>[8x]MPVTNLAELDALVARVKAAQAEFATFSQEQVDKIFRAASLAANQARIPLAQMAVEESGMGIVEDKVIKNHFASEFIYNKYKDEKTCGILEEDDNLGTMTIAEPVGIICGIVPTTNPTSTAIFKSLISLKTRNGIIFSPHPRAKNSTNAAAKLVLDAAIAAGAPKDIIGWIDQPSVELSNALMKHDGIALILATGGPGMVKAAYSSGKPAIGVGAGNVPVVIDETADIKRAVASILMSKTFDNGVVCASEQAAIVVSEVYDEVKERFATHKAHVLSKA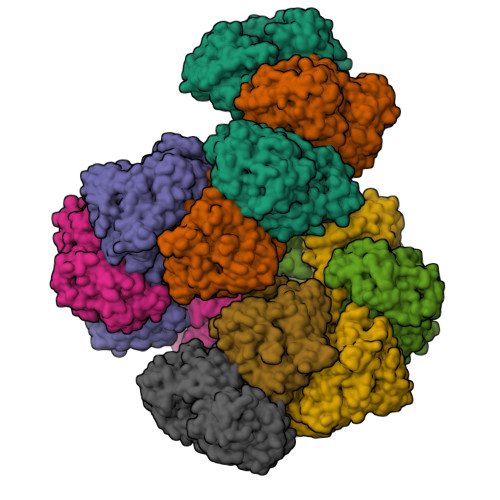DADKVRKVLLIDGALNAKIVGQPAAAIAEMAGVKVPADTKVLVGEGLGKVSYDDEFAHEKLSPTLGLFRADNFEDAVAQAVTMVEIGGIGHTSGLYTNQDVNADRIRYFGDKLKTARILVNIPTTHGGIGDLYNFNVAPSLTLGCGSWGGNSISENVGPKHLINKKTVAKRAENMLWHKLPKSIYFRRGSLPIALSDLEGKKRAFLVTDRFLFNNGYADDVVALLKAQGMEVQTFFEVEADPTLSVVEKGAAAMQSFQPDVILALGGGSPMDAAKIMWVMYEHPDTHFEELAMRFMDIRKRIYKFPKMGKKAELVCITTTSGTGSEVTPFAVVTDDKTGAKYPLADYELTPQMAIVDANLVMNMPKSLTAFGGYDAVTHALEAYVSVLANEYSDGQALQALKMLKEYLPSSYANGAKDPIAREKVHNAATIAGIAFANAFLGVCHSMAHKIGAEFHLPHGLANALLIANVVRYNANDNPTKQTAFSQYDRPQARRRYAEVADHLGLSQPGDRTAQKIERLLTWLDELKVNLDIPKSIQAAGVAEADFLAKVDELAVEAFDDQCTGANPRYPLIAELKEVLLASYYGKPFVEGQTFEGTTVIVKKADQEAAKAPKAKK Recently, mutational screening analysis identified the chloroplast-localized HJ resolvase MOC1 that is essential for chloroplast nucleoid segregation in Chlamydomonas reinhardtii and Arabidopsis thaliana. MOC1 exhibits dimerization and an RNaseH fold, belonging to the retroviral integrase superfamily. Moreover, we characterize a base recognition loop (BR loop) that protrudes into the junction and disrupts the C–G base pairs at the crossover. Residue D183 from the BR loop recognizes the cytosine, determining the cytosine-dependent HJ resolution.

We first determined the crystal structure of HJ-free ZmMOC1 (T107-V280) via iodide-based single-wavelength anomalous diffraction (I-SAD) at a refined resolution of 2.5 Å and the structure of a quadruple mutant NtMOC1 (N108-S275, I112V/Q162K/E235Q/239Q) at a 2.0 Å resolution. For each protomer, the core of NtMOC1 is formed by five-stranded β-sheets (β1β2β3β6β7) composed of three antiparallel (β1β2β3) and two parallel strands (β6β7)—a characteristic feature of the RNase H fold, belonging to the retroviral integrase superfamily. The β-sheets are flanked by six α helices (α1 and α2 on one side, and α3, α4, α5 and α6 on the other side). The α-helix 2 (α2) from each protomer constitutes a helical bundle, where G192, G196, G200, and A204 form a hydrophobic patch on the dimer interface. Both analytical ultracentrifugation (AUC) and size-exclusion chromatography (SEC) experiments revealed that double mutations of G200E and A204E could disrupt dimer formation. A structural homolog search by Dali40 revealed that NtMOC1 has the highest structural similarity with RuvC resolvase. NtMOC1 in the complex also exhibits dimerization, and the HJ is embedded into the cleft of the dimeric NtMOC1. Structural alignment of the apo NtMOC1 with HJ-bound NtMOC1 revealed minor conformational changes with an RMSD value of 0.527 Å over 242 Cα, which mainly arose from the loop preceding α2 (we termed this loop the base recognition loop (BR loop), discussed below). Mutation of Y180 (Y180A) has little effect on HJ binding and resolution activity. Although the overall structures of apo and HJ-bound NtMOC1 exhibited similar architectures, residues Y180 and D183 in the BR loop underwent striking conformational changes, demonstrating the great flexibility of the BR loop.

> AHMNAGWVIGVDPDTSGALALLKPNQPPQVFDSPHLKVLVGKGVRKRLDAKAIVQLLKSFEAPIGTTVYVEQSTPYPQDGKQGWWSGGFGYGMWIGILVASGFSVIPVPSSAWKSEFQLTKERSNKDYSRQVASQLFPSLSSLLKRKKDHGRAEALLIAAYGKGIKINSDS>[8x]DLILPFYKAGKVSFYQGDLDVLINFLEPD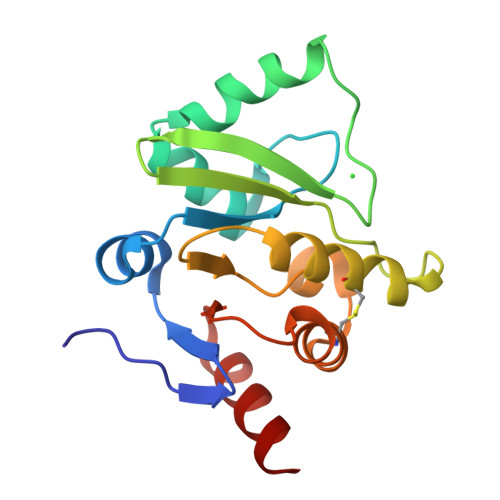VLVNAANGDLRHVGGVARAIDVFTGGKLTKRSKEYLKSSKAIAPGNAVLFENVLEHLSVLNAVGPRNGDSRVEGKLCNVYKAIAKCDGKILTPLISVGIFKVKLEVSLQCLLKTVTDRDLNVFVYTDQERVTIENFFNG>MSKPKISLTKGKHPCTFCQARKVKCDRSLPACQNCIERNVTELCEYDDNGSRKRARLADDVNLYDKKLFNIWNQYERLWIHDTLGQCQQGVYMGIAFPLDVSEYNNTKDFYGYECLFSKESIFKILDHSLERLGWLYFGFFTDISELPYQMERYWNEYESMNINLENEEATTRQTTFKKSADQILWDLVLRSVIVMTIYYMPAKSILSLVDIDAIEKYPLDFSESNEGVDELKKKYEIFDYCLRHTLNKVLRTIFTLPPDVRTLQIFLILSNTNFLQIYPSLGNNILVHCIHLAKVLGIKDFKLKINDSGSTRLQKLSMHNIWFRLSTVDYMRSSPNKIIALHTDNSSALTRKTLFTHCSI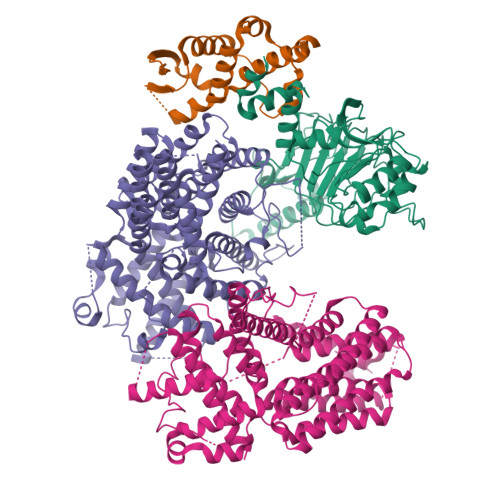DSIDVYDVESNLEVLRWKITSLDRDLEVSEPSLKTLKAMKELLGLLDRKTSVSNDASFNTKFESFFLKLQCNFVMWKILRYEFMQYGVTNGLQKLCCPARRIIALVANFLKEDYFEYTTHPFCVHILCVIAGFFSFYCIFHEADEVRDLRNDAVGLLKLLFDPLRPVISCFFSNLSRLEELRHIWKSVEITDQANRLVHPVMYVLKTDIIKLKRNLEIISGSLKDANYQETFKDKLEIDINTPALSSDFLEVVREFNLSHPLDINGKMSRQNN[2x];> MFDTKLFLSLPIDIRYTVYFFLGDVVQNVRPPAKSDIFNDELIAYPNIREFNQSLVDKYSKHIGVYDYIPNFIPNWCRDFDLLRHDIILTDRLRVCLQYEEQWFSVQWIVVSGELEIGIFTTDEQFLQVSYTINEYCHLLSIAQQDLRLGINVSDINDVNELCKEIQHRWLFDTVSYISFINCWDLDHENVVSIIPCMESFNNLHMLRIESKNMFNNLINTQGVRENPGKTIVYNVRQNIFELELYTLRDLGYKSVVDLQKWEQLQCLSLSGCEFIDLNNLILPQHCKMLILKEVKYIIWWDLSHLLKRIRPQWIINGQVKKPTKKEEEEESEWYNLYLEVVQTYQPLNFIELHNAKRVKGNLILPARLVTESRIKISNGTKVDSVLLI;> MSKENQNVVLVSVEGERFVVDRKIAERSLLLKNYLQDLNSGDLHDDNDADDDEDDEEDGDDEIVMPVPNVRSSVLQKVIEWAVHHKDSNFPDEDDDDSRKAAPVDPWDREFLKVDQEMLYEIILAANYLNIKPLLDAGCKVVAEMIRGRTPEEIRRTFNIVNDFTPEEEAAIRRENEWAEDR>[2x]MALSLYEKMLHKGMIIKNSNVYEKIKEIDTIIFDKTGTLTYGTPIVTQFIGDSLSLAYAASVEALSSHPIAKAIVKYAKEQGVKILEVKDFKEISGIGVRGKISDKIIEVKKAENNNDIAVYINGEPIASFNISDVPRPNLKDYLEKLKNEGLKIII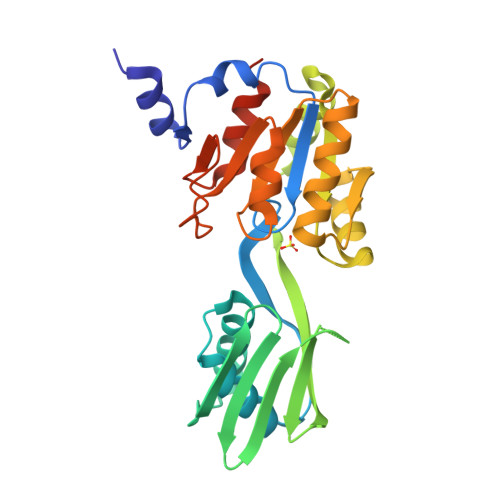LSGDKEDKVKELSKELNIQEYYSNLSPEDKVRIIEKLKQNGNKVLMIGDGVNDAAALALADVSVAMGNGVDISKNVADIILVSNDIGTLLGLIKNRKRLSNAIPSN> GPGSMEEHTEAGSAPEMGAQKALIDNPADILVIAAYFLLVIGVGLWSMCRTNRGTVGGYFLAGRSMVWWPVGASLFASNIGSGHFVGLAGTGAASGLAVAGFEWNALFVVLLLGWLFAPVYLTAGVITMPQYLRKRFGGRRIRLYLSVLSLFLYIFTKISVDMFSGAVFIQQALGWNIYASVIALLGITMIYTVTGGLAALMYTDTVQTFVILGGACILMGYAFHEVGGYSGLFDKYLGAATSLTVSEDPAVGNISSFCYRPRPDSYHLLRHPVTGDLPWPALLLGLTIVSGWYWCSDQVIVQRCLAGKSLTHIKAGCILCGYLKLTPMFLMVMPGMISRILYPDEVACVVPEVCRRVCGTEVGCSNIAYPRLVVKLMPNGLRGLMLAVMLAALMSSLASIFNSSSTLFTMDIYTRLRPRAGDRELLLVGRLWVVFIVVVSVAWLPVVQAAQGGQLFDYIQAVSSYLAPPVSAVFVLALFVPRVNEQGAFWGLIGGLLMGLARLIPEFSFGSGSCVQPSACPAFLCGVHYLYFAIVLFFCSGLLTLTVSLCTAPIPRKHLHRLVFSLRHSKEEREDLDADEQQGSSLPVQNGCPESAMEMNEPQAPAPSLFRQCLLWFCGMSRGGVGSPPPLTQEEAAAAARRLEDISEDPSWARVVNLNALLMMAVAVFLWGFYA;> MSALSLLILGLLTAVPPASCQQGLGNLQPWMQGLIAVAVFLVLVAIAFAVNHFWCQEEPEPAHMILTVGNKADGVLVGTDGRYSSMAASFRSSEHENAYENVPEEEGKVRSTPM

Human (h)SGLT1 and hSGLT2 are responsible for reabsorption of glucose in the proximal tubules after filtration through the glomerulus. SGLT2, a transmembrane protein with 14 helices and expressed specifically in the kidneys, has 60% sequence homology to SGLT1, which is also expressed in the small intestine. SGLT2 inhibitors that suppress glucose reabsorption and promote urinary excretion are considered a promising therapeutic tool to manage blood glucose levels in patients with type-2 diabetes. In this Article, we performed cryo-EM single-particle analyses to determine the structures of the genuine hSGLT2–MAP17 complexes with five inhibitors (canagliflozin, dapagliflozin, TA-1887, sotagliflozin and phlorizin).

Unexpectedly, phlorizin was found to bind to TM1, TM5 and TM8 in an inward-open structure, in contrast to the outward-facing structure that we observed for the gliflozins. This binding site is located near the Na2 site, where Na+ binds to the outward-facing structure. The glucose moiety of phlorizin is bound to the bending site of the intracellular side of TM1, whereas the aglycon moiety, connected to the glucose moiety via an ether bond, is surrounded by the side chain comprising A69, S70, A73 and S74 of TM1, D201 of TM5, and R300 of TM6, extending toward the lipid membrane. The ether bond is unique to phlorizin, whereas the central aromatic ring of the gliflozins connects directly to the glucose moiety, causing rigidity that prevents binding to the inward-open structure. Furthermore, the inward-open structure does not exhibit density for IL0 between TM0 and TM1. Phlorizin at up to 5,000 nM did not saturate the hSGLT2-expressing membrane; it exhibited biphasic kinetics, indicating that phlorizin has two binding sites on hSGLT2 (high- and low-affinity sites). In the phlorizin-bound inward-open structure, the extracellular-binding site is abolished, suggesting that phlorizin can bind to only one of the sites (extracellular or intracellular). Under the conditions of our cryo-EM analysis (no Na+ gradient and 500 μM phlorizin), phlorizin bound to the low-affinity intracellular site. We therefore believe that our cryo-EM analysis revealed binding from the intracellular side. After sodium and glucose are released, the transporter forms an inward-open structure and phlorizin and phloretin bind to this structure, inhibiting glucose transport.>MALVDGFLELERSSGKLEWSAILQKMASDLGFSKILFGLLPKDSQDYENAFIVGNYPAAWREHYDRAGYARVDPVVSHCTQSVLPIFWEPSIFQTRKQHEFFEEASAAGLVYGLTMPLHGARGELGWLSLSVEAENRAEANRFMESVLPTLWMLKDYALQSGAGLAFEHPVSKPVVLTSREKE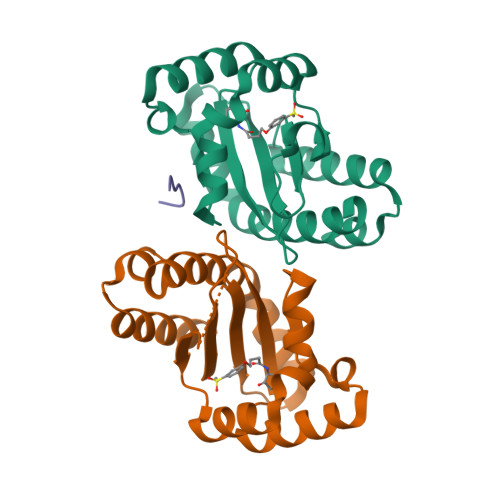VLQWCAIGKTSWEISVICNCSEANVNFHMGNIRRKFGVTSRRVAAIMAVNLGLITL[2x];> AHHHHA> MAHHHHHHMAKSGLRQDPQSTAAATVLKRAVELDSESRYPQALVCYQEGIDLLLQVLKGTKDNTKRCNLREKISKYMDRAENIKKYLDQEKEDGKYHKQIKIEENATGFSYESLFREYLNETVTEVWIEDPYIRHTHQLYNFLRFCEMLIKRPCKVKTIHLLTSLDEGIEQVQQSRGLQEIEESLRSHGVLLEVQYSSSIHDREIRFNNGWMIKIGRGLDYFKKPQSRFSLGYCDFDLRPCHET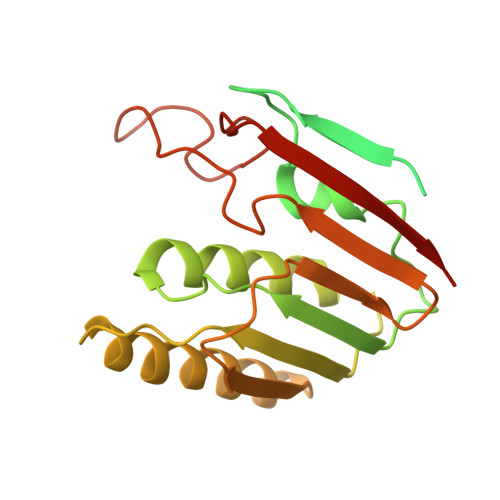TVDIFHKKHTKNI> MNYTKFDVKNWVRREHFEFYRHRLPCGFSLTSKIDITTLKKSLDDSAYKFYPVMIYLIAQAVNQFDELRMAIK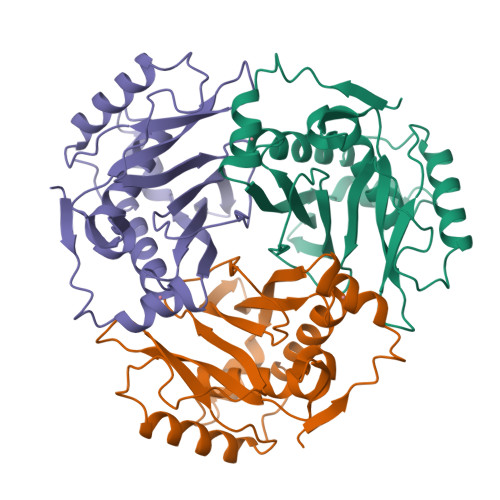DDELIVWDSVDPQFTVFHQETETFSALSCPYSSDIDQFMVNYLSVMERYKSDTKLFPQGVTPENHLNISALPWVNFDSFNLNVANFTDYFAPIITMAKYQQEGDRLLLPLSVQVHHAVCNGFHVARFINRLQELCNSKLK> MKITTWNVNSLNVRLPQVQNLLADNPPDILVLQELKLDQDKFP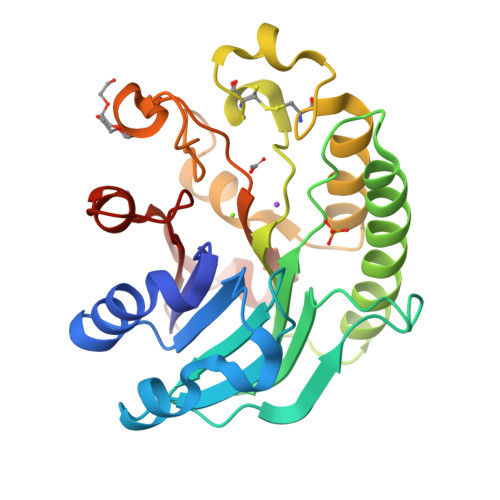AAALQMMGWHCVWSGQKTYNGVAIVSRSVPQDVHFGLPALPDDPQRRVIAATVSGVRVINVYCVNGEALDSPKFKYKEQWFAALTEFVRDEMTRHGKLVLLGDFNIAPADADCYDPEKWHEKIHCSSVERQWFQNLLDLGLTDSLRQVHPEGAFYTWFDYRGAMFQRKLGLRIDHILVSPAMAAALKDVRVDLETRALERPSDHAPVTAEFDW> GAGCAGACCTG;> ACGCCACTCA;> CACGT;> TCTGAGTGGGGTCTGC

In this work, we exhaustively probe the ability of all 36 immobile HJ sequences to form DNA crystals in two different designed systems. Three separate self-assembling DNA crystal systems are described in this report: the “4 × 5” and “4 × 6” designs (collectively referred to as the 4 × N systems), and a third construct with a “scrambled” sequence variant of the 4 × 6 lattices. Self-assembly was mediated by three constituent oligonucleotides: (S1) containing four sequence repeats of either 5 or 6 bases; (S2) composed of 21 bases containing complementary regions to both (S1); and (S3) which forms the second junction crossover. The HJ serves as the fundamental component at the core of each unit, and the ultimate assembly of the full lattice is facilitated by the complementary 2-base sticky ends that tail each duplex.

The 4 × 5 system robustly crystallized with 75% of the junctions, and we obtained crystals in all but 9 of 36 sequences. Of the resulting structures, 18 exhibited P32 symmetry with average cell dimensions a = b = 68.85 Å c = 60.09 Å, with only nine retaining the original P3221 symmetry with average cell edges a = b = 68.17 Å c = 60.60 Å. Although the cell parameters between the two symmetries were virtually indistinguishable, the differences between the periodicity of the lattices is dramatic, with vastly different cavity sizes. We hypothesize that even a small difference in junction angles could have a significant global effect on the assembly of the lattice, thereby eliminating the strain in the P3221 lattices.>MATDWTDNRKNLMLFAGRAHPELADQVAKELDVAVTAQTARDFANGEIFVRFDESVRGCDAFVLQSHPAPLNQWLMEQLIMIDALKRGSAKRITAILPFYPYARQDKKHRGREPISARLVADLLKTAGADRIVSVDLHTDQIQGFFDGPVDHMRAQKLLTGYIGEHYADEDMVVVSPDSGRVRVAEKWADSLGGVPLAFIHKTRDPLVPNQVKSNRVVGDVKGKTCILTDDMIDTGGTIAGAVNLLREDGAKDVIIAATHGVLSDPAPQRLAECGAREVIVTNTLPITEDKRFPQLTV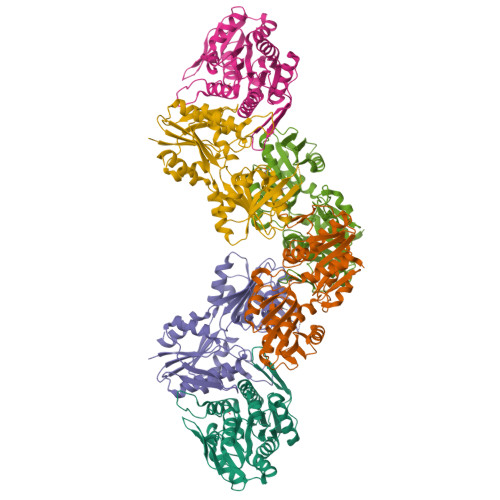LSIAPLLANTIRAVFENGSVTGLFDGSA[3x]9-amino-5-(2-aminopyrimidin-4-yl)pyrido[3',2':4,5]pyrrolo[1,2-c]pyrimidin-4-ol 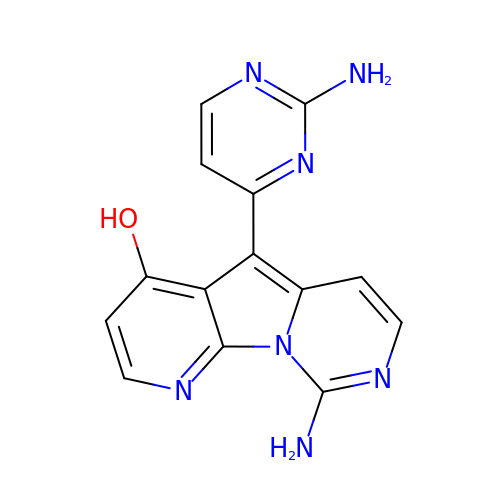| C14 H11 N7 O | RTHKPHCVZVYDFN-UHFFFAOYSA-N>MFENITAAPADPILGLADLFRADERPGKINLGIGVYKDETGKTPVLTSVKKAEQYLLENETTKNYLGIDGIPEFGRCTQELLFGKGSALINDKRARTAQTPGGTGALRVAADFLAKNTSVKRV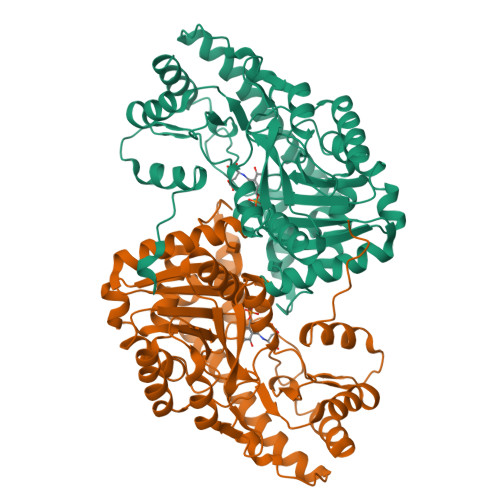WVSNPSWPNHKSVFNSAGLEVREYAYYDAENHTLDFDALINSLNEAQAGDVVLFHGCCHNPTGIDPTLEQWQTLAQLSVEKGWLPLFDFAYQGFARGLEEDAEGLRAFAAMHKELIVASSYSKNFGLYNERVGACTLVAADSETVDRAFSQMKAAIRANYSNPPAHGASVVATILSNDALRAIWEQELTDMRQRIQRMRQLFVNTLQEKGANRDFSFIIKQNGMFSFSGLTKEQVLRLREEFGVYAVASGRVNVAGMTPDNMAPLCEAIVAVL[2x]>GQSNSNNWRWFDDRSGRWCSY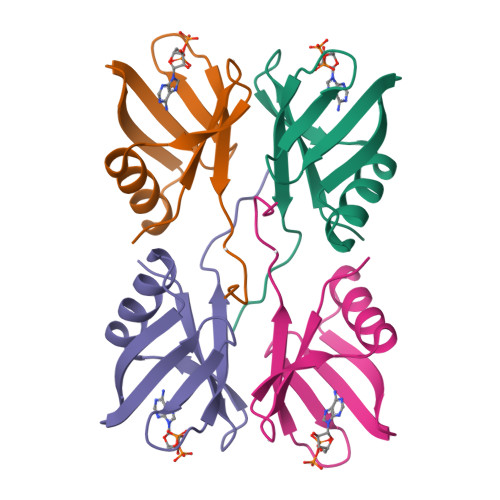SASNNSTIDSAWKSGETSVRFTAGRRRYTVQFTTMVQVNEETGNRRPVMLTLLRVPRLNKNSKNSNGQEL[2x]> GPHMCAFHAKFKEAALFKRVVESLKSTIDKTNFDCSDAGIAVQCMDNSHVSLVSLLIETDAFDEFQCLKPITLGINLTHLSKILKALDNDCGLILDVKKVDDAVLSITSEGTNKTMKFGLNLVDIEAESVEIPELQSDAIITLSSAEFLKITKDFSALGDDSITIGCTKNEVTLTTKGAMCETCMT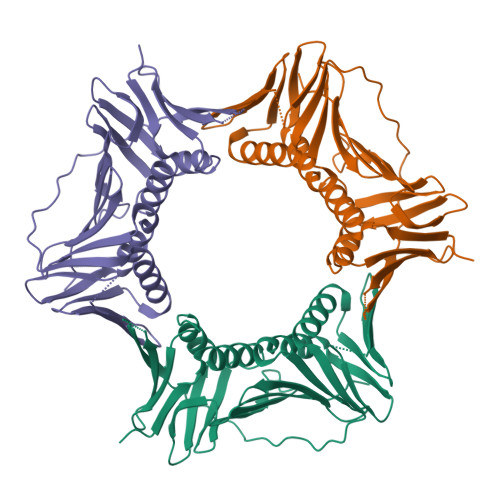LSALENVDSNGLQIEHNKDVTASFALKQISEFAKSAPLADNVKLSLSGQAPLIMEFKGEACVLKFYLAPKFDEEDEPQE>[3x]QFVDMSPASNNSECLDSQVDAAAFSKLMRPYPIDPAKVDGIIYPLGRTYSNITLAYTGLFPLQGDLGTQYLYSASHAVGNDGDPTKAYISNYSLLVNDFDNGFVVRVGAAANSTGTIVISPSVQTKIKKAYPAFILGSSLTNTSAGQPLYANYSLTIIPDGCGTVLHAFYCILKPRTGNRCPGGSGYNAYFIYETIHNDCNSAINKNASLNSFKSFFDLVNCTFFNSWDITADEVKEWFGITQDTQGVHLYSSRKGDLYGGNMFRFATLPVYEGIKYYTVIPRSFRSKANRREAWAAFYVYKLHQLTYLLDFSVDGYIRRTIDCGHDDLSQLHCSYTSFEVDTGVYSVSSYEASAIGTFIEQPNATECDFSPMFKGVAPQVYNFKRLVFSNCNYNLTKLLSLFAVDEFSCNGISPDAIARGCYSTLTVDYFAYPLSMKSYIRPGSAGNIPLYNYKQSFAHPTCRVLASVPPNVTITKPEAYGYISKCSRL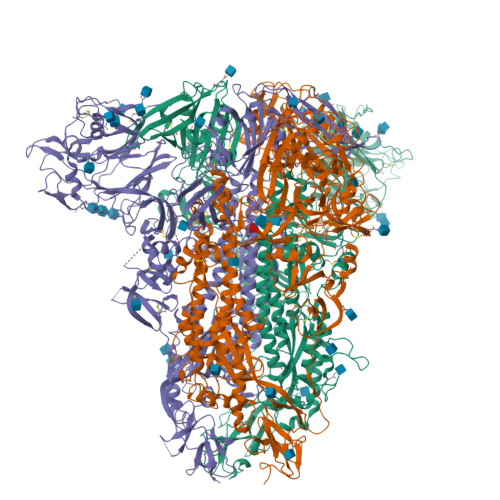TGDYQHIETPLYINPGEYSICRDFAPLGFSEDGQVFKRTLTQFEGGGLLIGVGTRVPMTANLEMGFVISVQYGAGTDSVCPMLDLGESSTITNRLGKCVDYSLYGVTGRGVFQNCTAVGVKQQRFVYDSFDNLVGYYSDDGNYYCVRPCVSVPVSVIYDKSTNLHATLFGSVACEHVTTMMSQFSRLTQSNLRRRDSNAPLQTAVGCVIGLSNNSLVVSECKLPLGQSLCAVPSVSLFRSYSASQFQLAVLNYTSPIVLTPINSSGFTAAIPTNFSFSVTQEYIETSIQKVTVDCKQYVCNGFTRCEKLLVEYGQFCSKINQALHGANLRQDESVYSLYSNIKTTSTQTLEYGLNGDFNLTLLQVPQIGGSPSGYRSAIEDLLFDKVTIADPGYMQGYDDCMKQGPQSARDLICAQYVSGYKVLPPLYDPNMEAAYTSSLLGSIAGAGWTAGLSSFAAIPFAQSMFYRLNGVGITQQVLSENQKLIANKFNQALGAMQTGFTTSNQAFSKVQDAVNANAQALSKLASELSNTFGAISSSISDILARLDTAEQDAQIDRLINGRLTSLNAFVSQQLVRSETAARSAQLASDKVNECVKSQSKRNGFCGSGTHIVSFVVNAPNGFYFFHVGYVPTNYTNVTAAYGLCNNNNPPLCIAPIDGYFITNQTTTYSVDTEWYYTGSSFFKPEPITQANSRYVSSDVKFEKLENNLPPPLLE In this study, we co-crystalized ELIC with the general anesthetic isoflurane, which is known to inhibit mammalian neuronal and muscle nAChRs3132 and GLIC33. The crystal structures of ELIC-isoflurane were determined with resolutions of 3.0 Å and 3.4 Å in the absence and presence of agonists, corresponding to the presumed resting and desensitized states of ELIC, respectively. As a homolog to eukaryotic pLGICs, ELIC shares similar pharmacological profiles of eukaryotic cation-conducting pLGICs with respect to modulation by general anesthetics. Thus, isoflurane inhibition via a direct pore-binding mechanism is likely accomplished jointly by stabilizing the closed channel conformation and blocking the open channel.

For ELIC crystallized in the presence of both isoflurane and the agonist BrPPA (presumed in a desensitized state), the FO-FC omit electron density map also indicates double isoflurane occupancies in the pore. The bromine atom of the agonist BrPPA co-crystalized with ELIC produced bromine-specific anomalous signals in the X-ray diffraction data collected with a wavelength near the K-edge peak of Br (0.9199 Å). The anomalous signals and FO-FC electron densities revealed BrPPA binding sites behind loop C and nearby loop A in the extracellular domain. These sites were reported previously to bind agonists, competitive antagonists, and modulators in ELIC404142 and in other pLGICs4344. The observation of isoflurane in the pore of ELIC under desensitization conditions could be attributed to an open pore-blocking mechanism. By this mechanism, isoflurane occupies and occludes an open pore and then remains in the pore when the channel desensitizes. In contrast, isoflurane molecules in the modeled desensitized pore moved away substantially from their initial positions and deviated from the center of the pore. In contrast, mobile isoflurane molecules inside the desensitized pore increased the RMSF of the pore region.

>[10x]APADNAADARPVDVSVSIFINKIYGVNTLEQTYKVDGYIVAQWTGKPRKTPGDKPLIVENTQIERWINNGLWVPALEFINVVGSPDTGNKRLMLFPDGRVIYNARFLGSFSNDMDFRLFPFDRQQFVLELEPFSYNNQQLRFSDIQVYTENIDNEEIDEWWIRGKASTHISDIRYDHLSSVQPNQNEFSRITVRIDAVRNPSYYLWSFILPLGLIIAASWSVFWLESFSERLQTSFTLMLTVVAYAFYTSNILPRLPYTTVIDQMIIAGYGSIFAAILLIIFAHHRQANGVEDDLLIQRCRLAFPLGFLAIGCVLVIRGITL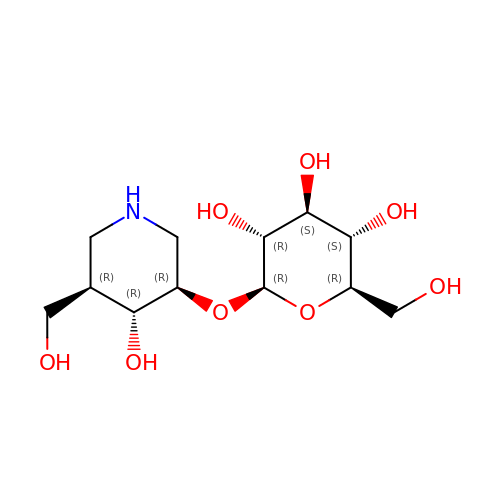(3R,4R,5R)-4-hydroxy-5-(hydroxymethyl)piperidin-3-yl beta-D-glucopyranoside | C12 H23 N O8 | BEXVSXHKIARRKH-FYKVHUBJSA-N>[3x]MRGSHHHHHHGSMPVAGSELPRRPLPPAAQERDAEPRPPHGELQYLGQIQHILRCGVRKDDRTGTGTLSVFGMQARYSLRDEFPLLTTKRVFWKGVLEELLWFIKGSTNAKELSSKGVKIWDANGSRDFLDSLGFSTREEGDLGPVYGFQWRHFGAEYRDMESDYSGQGVDQLQRVIDTIKTNPDDRRIIMCAWNPRDLPLMALPPCHALCQFYVVNSELSCQLYQRSGDMGLGVPFNIASYALLTYMIAHITGLKPGDFIHTLGDAHIYLNHIEPLKIQLQREPRPFPKLRILRKVEKIDDFKAEDFQIEGYNPHPTIKMEMAV

Thymidylate synthase (TS, EC 2.1.1.45) is a ubiquitous enzyme that catalyzes the reductive methylation of 2′-deoxyuridine-5′-monophosphate (dUMP) to 2′-deoxythymidyne-5′-monophosphate (dTMP) using N5,N10-methylenetetrahydrofolate (mTHF) as a cofactor. In cells, TS provides the only synthetic source of dTMP necessary for DNA biosynthesis. TS works as an obligate homodimer, having residues from both enzyme subunits that contribute to substrate binding in each catalytic site. TS subunits are characterized by two domains, known as large and small domains (LD and SD, respectively).

The structure of hTS in complex with the substrate analogue FdUMP (Ki of 1.1 nM) was determined to 2.08 Å resolution. In both complexes, the two subunits of the hTS homodimer adopt the active conformation, showing that Cys195 is exposed to the catalytic cavity, as occurs in previously reported structures. FdUMP fully occupies the hTS active site, perfectly mimicking the interactions entailed by dUMP in the substrate pocket. The 5-fluorine of FdUMP forms an additional water-mediated interaction with the Tyr135 hydroxyl. FdUMP C6 is positioned 3.09–3.29 Å away from the Cys195 thiol, which is the same distance observed in the dUMP complex. On the other hand, in our complex, FdUMP mimics the substrate, placing its 5-fluoro-uracil C6 in an optimal position to form the covalent adduct with the reactive thiol of Cys195. In contrast, in the hTS complex, the FdUMP uracil is shifted far from the isostructural Tyr135, and a water molecule mediates its interaction with the fluorine of the inhibitor. A comparison of EfTS and hTS complexes shows that, in hTS, the orientation of His196 prevents the inhibitor from lying closer to Tyr135, whereas in EfTS, the sidechain of His198 (corresponding to hTS His196) is rotated by ~70°, allowing the direct interaction between the fluorine and Tyr145. The superimposition further evidences that FdUMP in hTS partially overlaps the cofactor site of EfTS.>[6x]GNMEASEVMKE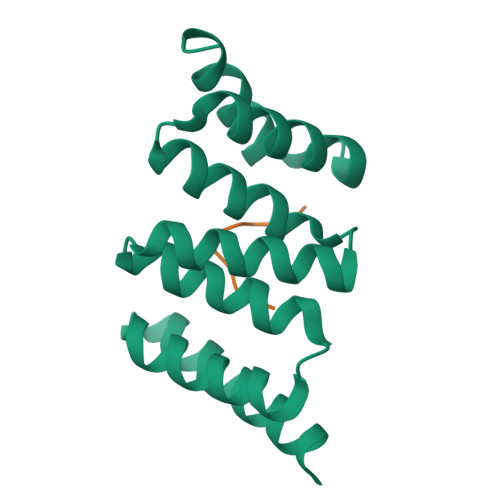KGNAAYKGKQWNKAVNFYTEAIKLNGANATYYCNRAAAFLELCCFQQAEQDCTKAMLIDKKNVKAYLRRGTARESLVRYKEAAADFRHALVLEPQNKTAKVAEKRLRKHI;>GSKMEEVD[6x]>[4x]EQAVERQGRPVLLLPSFPTPNGELHLGHLSGPFLNADACRRALLAAGERAHLLLGTVGHQSQVSAAAEAEGLSFHELAERNTDAIIEGLQAAGIDWDVFVRPSEPAYPAMATSVFESLRDRGVLVRRTEPTNYCEPCGRFLLEAFVAGHCPHCGSNQTAGIECELCALPYDDRDLVDPSCATCGAAATQRPLTRYFMP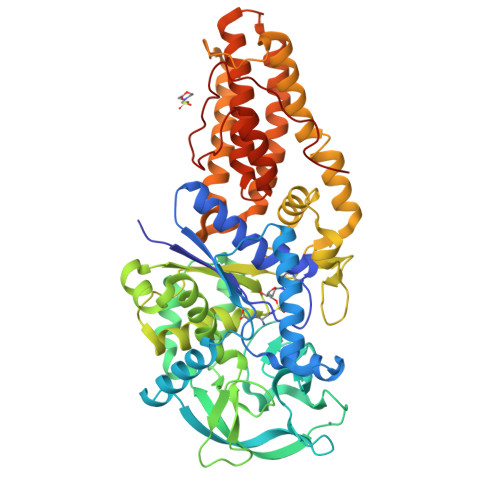LEPLRDELSGYLRGAAMHGRLRAYTERVLAKTLPDLPVSIPAEHGIPIHVEDASGPAEQRMYSAFELAARFLTALDGFADGWEAYARQENPRTVLFFGFDNAFLRAFAFPAVLGAFTDALPLPEALVCNDFYLLDGEKFSTGRKHAVWARQAVTPANADQLRLYLAATSPDVRRRDFTTRGYAEFVTAELIGRWQRRLDDVGGRVAEHFGGLTPEAGGWHAEAERFYGQIKEFASCATLDYLPGRFKPRAVVAAACAFIRQAEDFAEVSADATPGSGIARTCAALELMALRTLAMAVWPLAPEFGRRVAAALGEDTIALEPTPRWVRPDTEIKFATDHFSPDEVVAGR> QPP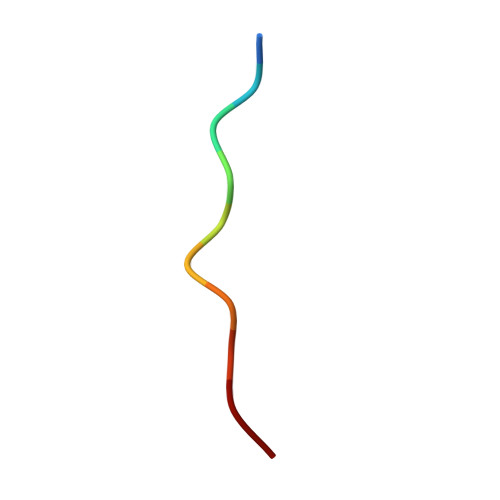VPPQRPM> MGWVPDEWSIDHDTLIDAGGYVQKLKLYPYFDAAHYVLTCLSVRHDLGPDAISFSRKHPFSCWLSCMLMSFAGSFLSCFLLGEPIISPLKQHADILLGSIVWYLVFYSPFDVVFRLATWFPVKLGLSVLKEVQRTHKIAAGVKHAVRIYPESYLVQILVGVAKGAGSGVVKIVEQLARGTWHPTNHEILRPSFTTKACVIASIVFTL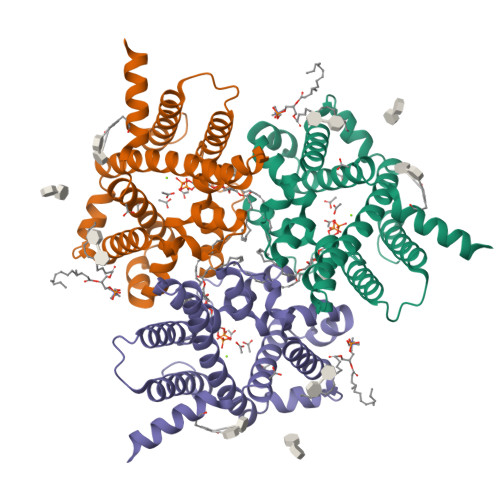ERHSMYVTAPHDLVYLCVVGFFIYFKLASLCLSVHDVLMPIENVLHHHHHH>MDLKILSLATDKTTDKLQEFLQTLKDDDLASLLQNQAVKGRAVGTLLRAVLKGSPCSEEDGALRRYKIYSCCIQLVESGDLQQDVASEIIGLLMLEVHHFPGPLLVDLASDFVGAVREDRLVNGKSLELLPIILTALATKKEVLACGKGDLNGEEYKRQLIDTLCSVRWPQRYMIQLTSVFKDVCLTPEEMNLVVAKVLTMFSKLNLQEIPPLVYQLLVLSSKGSRRSVLDGIIAFFRELDKQHREEQSSDELSELITAPADELYHVEGTVILHIVFAIKLDCELGRELLKHLKAGQQGDPSKCLCPFSIALLLSLTRIQRFEEQVFDLLKTSVVKSFKDLQLLQGSKFLQTLVPQRTCVSTMILEVVRNSVHSWDHVTQGLIEFGFILMDSYGPKKILDGKAVEIGTSLSKMTNQHACKLGANILLETFKIHEMIRQEILEQVLNRVVTRTSSPINHFLDLFSDIIMYAPLILQNCSKVTETFDYLTFLPLQTVQGLLKAVQPLLKISMSMRDSLILVLRKAMFASQLDARKSAVAGFLLLLKNFKVLGSLPSSQCTQSIGVTQVRVDVHSRYSAVANETFCLEIIDSLKRSLGQQADIRLMLYDGFYDVLRRNSQLASSIMQTLFSQLKQFYEPEPDLLPPLKLGACVLTQGSQIFLQEPLDHLLSCIQHCLAWYKSRVVPLQQGDEGEEEEEELYSELDDMLESITVRMIKSELEDFELDKSADFSQNTNVGIKNNICACLIMGVCEVLMEYNFSISNFSKSKFEEILSLF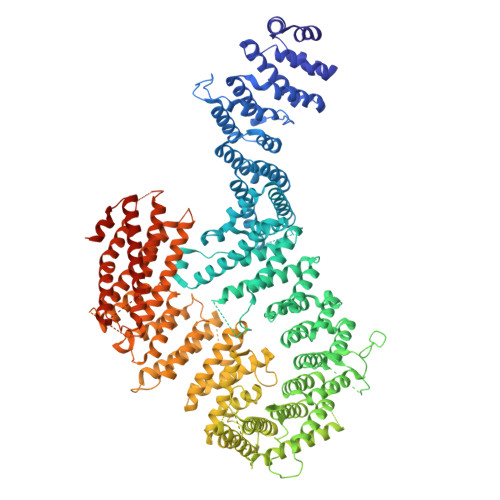TCYKKFSDILSEKAGKGKAKMTSKVSDSLLSLKFVSDLLTALFRDSIQSHEESLSVLRSSGEFMHYAVNVTLQKIQQLIRTGHVSGPDGQNPDKIFQNLCDITRVLLWRYTSIPTSVEESGKKEKGKSISLLCLEGLQKTFSVVLQFYQPKVQQFLQALDVMGTEEEEAGVTVTQRASFQIRQFQRSLLNLLSSEEDDFNSKEALLLIAVLSTLSRLLEPTSPQFVQMLSWTSKICKEYSQEDASFCKSLMNLFFSLHVLYKSPVTLLRDLSQDIHGQLGDIDQDVEIEKTDHFAVVNLRTAAPTVCLLVLSQAEKVLEEVDWLIAKIKGSANQETLSDKVTPEDASSQAVPPTLLIEKAIVMQLGTLVTFFHELVQTALPSGSCVDTLLKGLSKIYSTLTAFVKYYLQVCQSSRGIPNTVEKLVKLSGSHLTPVCYSFISYVQNKSSDAPKCSEKEKAAVSTTMAKVLRETKPIPNLVFAIEQYEKFLIQLSKKSKVNLMQHMKLSTSRDFKIKGSVLDMVLREDEEHHHHHH[4x]2,2'-iminodibenzoic acid | C14 H11 N O4 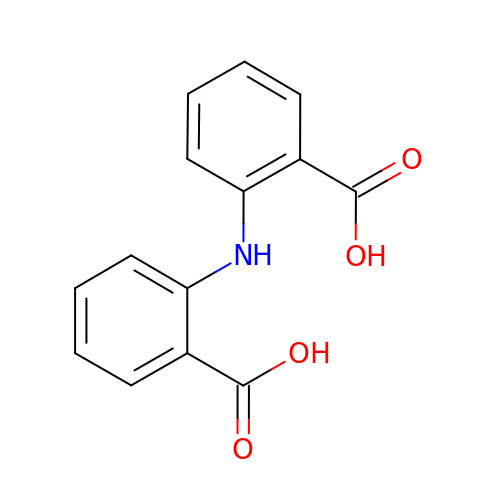| ZFRNOTZQUGWMQN-UHFFFAOYSA-N>GSHMLHWGPKYWRSLHLYAIFFSDAPSWKEKYEAIQWILNFIESLPCTRCQHHAFSYLTKNPLTLNNSEDFQYWTFAFHNNVNNRLN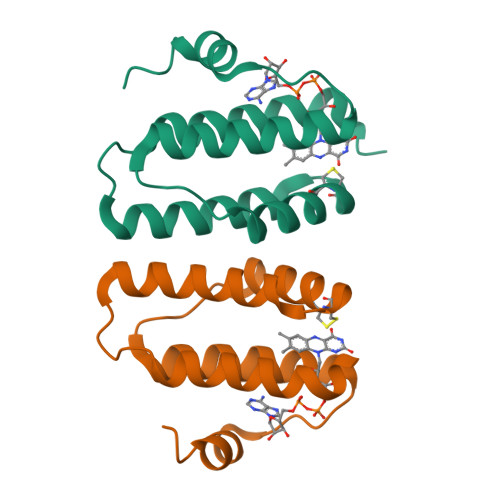KKIISWSEYKNIYEQSILK[2x]2-acetamido-2,3-dideoxy-D-ribo-hexitol 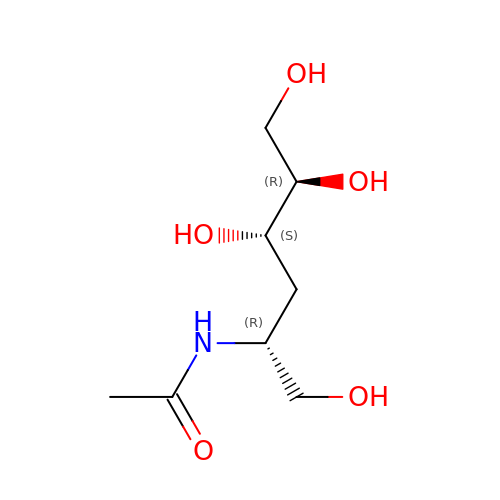| C8 H17 N O5 | LGGVICIJYZNZDM-GJMOJQLCSA-N2-({6-[(3R)-3-aminopiperidin-1-yl]-3-methyl-2,4-dioxo-3,4-dihydropyrimidin-1(2H)-yl}methyl)benzonitrile 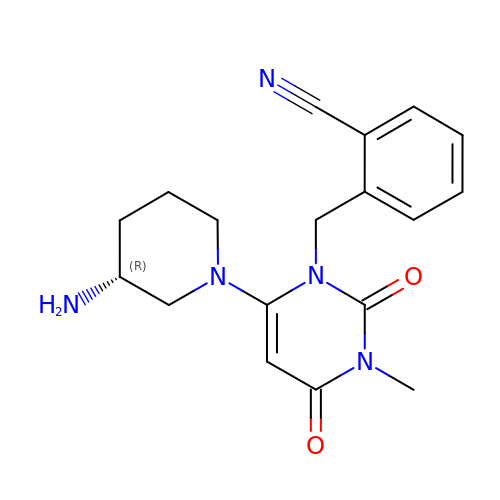| C18 H21 N5 O2 | ZSBOMTDTBDDKMP-OAHLLOKOSA-N> TPKKNISKGAVLHEKPMTVMVLTATEPFNYKEGKENMFHATVATESKYYRVKVFNMDLKEKFTENQFITISKYFNSSGILEINETATVSEAAPNQMFEVPKNIIRSAKETLKISKIKELDSGTLIYGVFAVEKKKVNDKSITFKIKDNEDNIKVVWDKEQHNINYEKGDKLQLFSFHLRKGNGKPILHSGNHSFI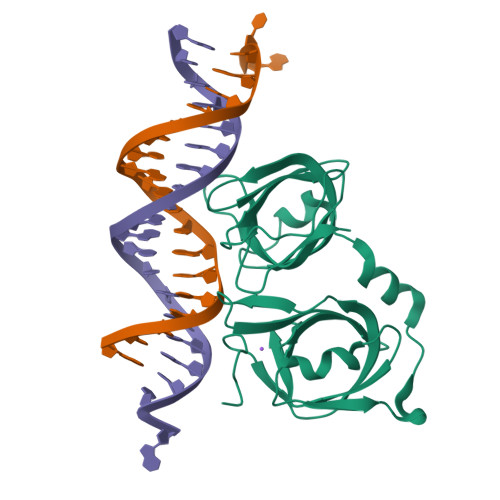KGE> SNMWVIGKSKAQDAKAIMVNGPQFGWYAPAYTYGIGLHGAGYDVTGNTPFAYPGLVFGHNGVISWGSTAGLGDDVDIFAERLSAEKPGYYLHNGKWVKMLSREETITVKNGQAETFTVWRTVHGNILQTDQTTQTAYAKSRAWDGKEVASLLAWTHQMKAKNWQEWTQQAAKQALTINWYYADVNGNIGYVHTGAYPDRQSGHDP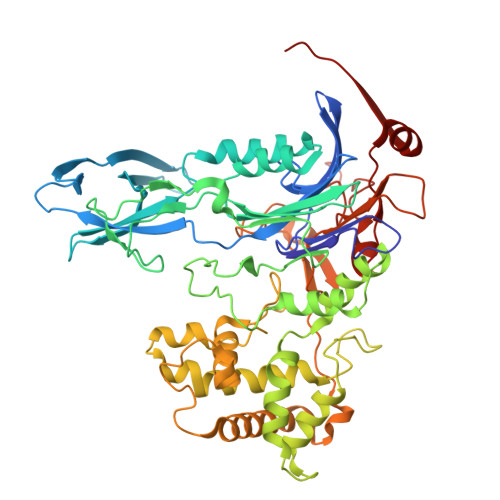RLPVPGTGKWDWKGLLPFEMNPKVYNPQSGYIANWNNSPQKDYPASDLFAFLWGGADRVTEIDRLLEQKPRLTADQAWDVIRQTSRQDLNLRLFLPTLQAATSGLTQSDPRRQLVETLTRWDGINLLNDDGKTWQQPGSAILNVWLTSMLKRTVVAAVPMPFDKWYSASGYETTQDGPTGSLNISVGAKILYEAVQGDKSPIPQAVDLFAGKPQQEVVLAALEDTWETLSKRYGNNVSNWKTPAMALTFRANNFFGVPQAAAEETRHQAEYQNRGTENDMIVFSPTTSDRPVLAWDVVAPGQSGFIAPDGTVDKHYEDQLKMYENFGRKSLWLTKQDVEAHKESQEVLHVQR>MQRDRDSSGSNARKGNRPPGLRGKDIGLYYRNLARQQKKDRGENAESKEPQIRLGCNVSAPSGVLERVKELMEDYSRAPSRQNVDDKNVDAKFQQQFRHLLSVNFEEFVAETKERNADLDWVNPKLDERLQLELGQRQLEENAKKRLEARKKLPTMKYADDIIQAVRENQVILIVGSTGCGKTTQVPQILLDDAISRGCASSCRIICTQPRRISAIAIAEWVSYERCESLGNSVGYQIRLESRKARERASITYCTTGVLLQQLQSDPLMHNLSVLILDEIHERSVETDLLMGLLKVILPHRPDLKVILMSATVREQDFCDYFNNCPMFRIEGVMFPVKMLYLEDVLSKTNYEFQKFRDRRPKRDPPERRMKHEAMIEPYLRRIRNSYDSRVLDKLRLPESEGCEDIDFIADLVYYICENEPEGAILVFLPGYDKISQLYNILDKPKTSKGQRWRDHMAVFPLHSLMQSGEQQAVFRRPPAGQRKVIISTIIAETSVTIDDVVYVINSGRTKATNYDIETNIQSLDEVWVTKANTQQRRGRAGRVRPGICYNLFSRAREDRMDDIPTPEILRSKLESIILSLKLLHIDDPYRFLQTLINAPNPEAIKMGVELLKRIEALDQTGTLTPLGMHLAKLPIDPQMGKMILMSALFCCLDPITSAAAALSFKSPFYSPLGKESRVDEIKRRMARNMRSDHLMVHNTIIAYRDSRYSHAERDFCYKNFLSSMTLQQLERMKNQFSELLYNYKFLASSNCKD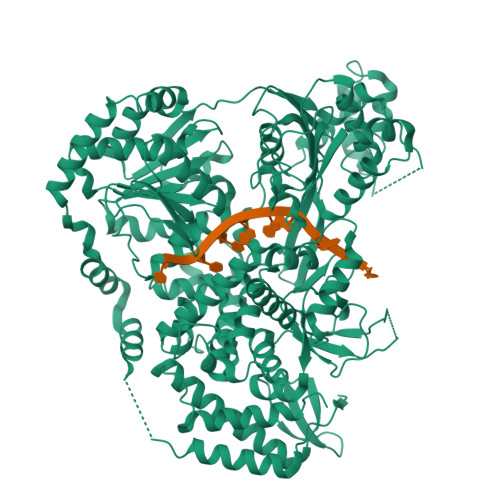AASNKNSEKIPLLRAIIGAGLYPNMAHLRKSRQIKNRVRAIHTMATDDGRRVNFHPSSVNSGESGFDSAYFVYFQRQKSTDLFLLDSTMVFPMALIIFGDGVEAGVTQNTPYLCVAKTYYFKCNRETADVVIQLRSNLEKLLLKKALYPAPIEENGYEKQLIKAIELLLSLDERLGEDYISSDEIDDIVD[2x]>[2x]AHHHHHHHHAAANTSYVDYNVEANPDLYPLCVETIPLSFPDCQNGPLRSHLICDESATPYDRAASLISLFTLDELIANTGNTGLGVSRLGLPAYQVWSAALHGLDRANFSDSGSYNWATSFPQPILTTAALNRTLIHQIASIISTQGRAFNNAGRYGLDVYAPNINTFRHPVWGRGQETPGEDVSLAAVYAYEYITGIQGPDPDSNLKLAATAKHYAGYDIENWHNHSRLGNDMNITQQDLSEYYTPQFHVAARDAKVHSVMCAYNAVNGVPACADSYFLQTLLRDTFGFVDHGYVSSDCDAAYNIYNPHGYASSQAAAAAEAILAG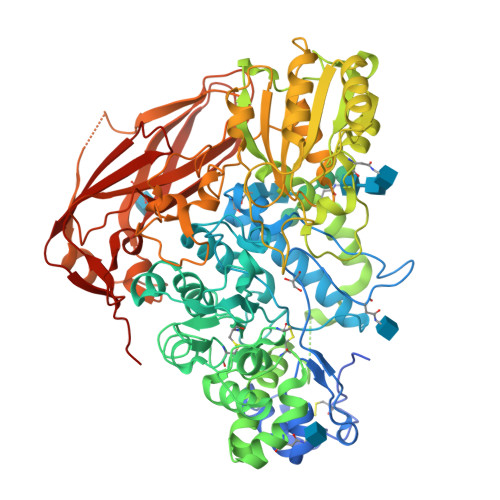TDIDCGTTYQWHLNESITAGDLSRDDIEKGVIRLYTTLVQAGYFDSNTTKANNPYRDLTWSDVVETDAWNISYQAATQGIVLLKNSNNVLPLTEKAYPPSNTTVALIGPWANATTQLLGNYYGNAPYMISPRAAFEEAGYNVNFAEGTGISSTSTSGFAAALSAAQSADVIIYAGGIDNTLEAEALDRESIAWPGNQLDLIQKLASSAGNKPLIVLQMGGGQVDSSSLKNNTNVSALLWGGYPGQSGGFALRDIITGRKNPAGRLVTTQYPASYAEEFPATDMNLRPEGDNPGQTYKWYTGEAVYEFGHGLFYTTFAESSSNTTTREIKLNIQDILSQTHEDLASITQLPVLNFTANIQNTGKVESDYTAMVFANTSDAGPAPYPVKWLVGWDRLGDVKVGETRELRVPIEVGSFARVNEDGDWVLFPGTFELGLNLERKVRVKVVLSGEEEVVLKWPGKE> MEEQNANQMLTDILSFMKS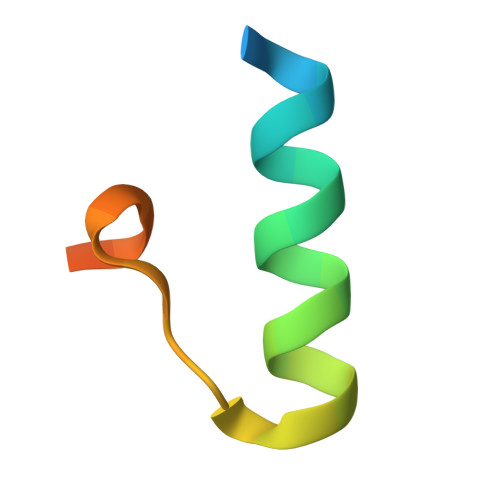GKRAAALEHHHHHH> AEEWYFGKITRRESERLLLNPENPRGTFLVRESETTKGAYCLSVSDFDNAKGLNVKHYKIRKLDSGGFYITSRTQFSSLQQLVAYYSKH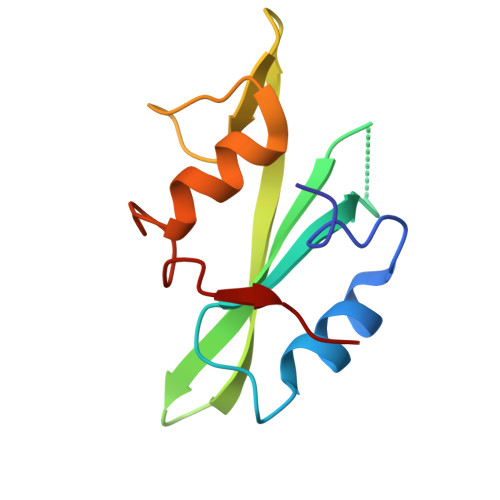ADGLCHRLTNVCPT2-({4-[(2-amino-4-oxo-4,7-dihydro-3H-pyrrolo[2,3-d]pyrimidin-5-yl)methyl]benzene-1-carbonyl}amino)-4-carbamoylbenzoic acid | C22 H18 N6 O5 | 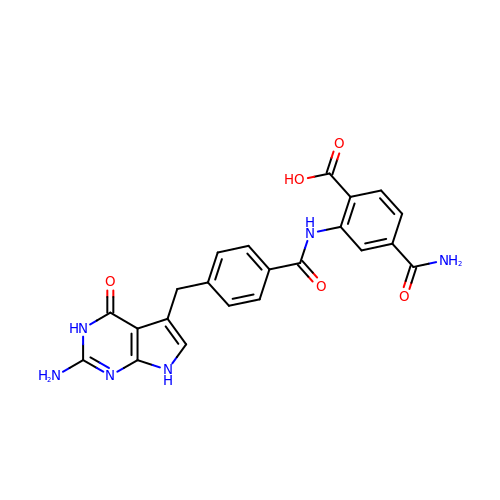ZFQOKUXSWWJOFS-UHFFFAOYSA-N>[4x]GSSPGTSNKRLRQVSSLVLHIEEAHKLPVKHFTNPYCNIYLNSVQVAKTHAREGQNPVWSEEFVFDDLPPDINRFEITLSNKTKKSKDPDILFMRCQ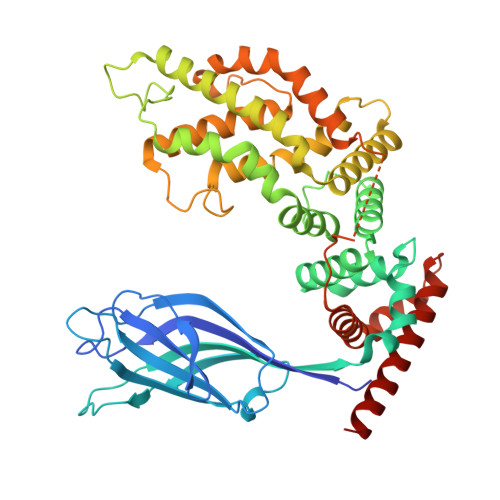LSRLQKGHATDEWFLLSSHIPLKGIEPGSLRVRARYSMEKIMPEEEYSEFKELILQKELHVVYALSHVCGQDRTLLASILLRIFLHEKLESLLLCTLNDREISMEDEATTLFRATTLASTLMEQYMKATATQFVHHALKDSILKIMESKQSCELSPSKLEKNEDVNTNLTHLLNILSELVEKIFMASEILPPTLRYIYGCLQKSVQHKWPTNTTMRTRVVSGFVFLRLICPAILNPRMFNIISDSPSPIAARTLILVAKSVQNLANLVEFGAKEPYMEGVNPFIKSNKHRMIMFLDELGNVPELPDTTEHSRTDLSRDLAALHEICVAHSDELRTLSNERGAQQHVLKKLLAITELLQQKQNQYTKTNDVR>PNFSGNWKIIRSENFEELLKVLGVNVMLRKIAVAAASKPAVEIKQEGDTFYIKVSTTVRTTEINFKVGEEFEEQTVDGRPCKSLVKWESENKMVCEQKLLKGEGPKTSWTLELTNDGELIETMTADDVVCT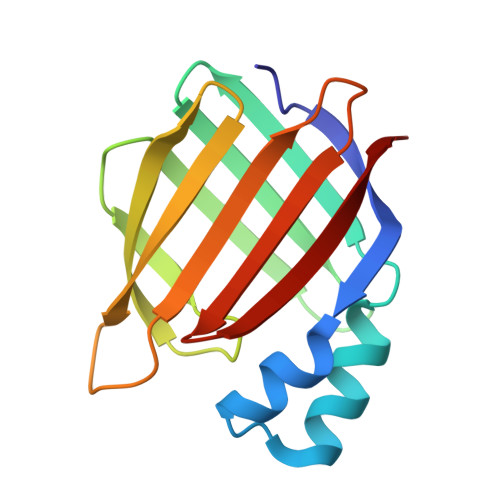KVFVRE[2x]>[2x]GMIKQDVICYEKEDVVKRNNINITGGGEKTVLLAHGFGCDQNMWRFMLPELEKQFTVIVFDYVGSGQSDLESFSTKRYSSLEGYAKDVEEILVALDLVNVSIIGHSVSSIIAGIASTHVGDRISDITMICPSPCFMNFPPDYVGGFERDDLEELINLMDKNYIGWANYLAPLVMGASHSSELIGELSGSFCTTDPIVAKTFAKATFFSDYRSLLEDISTP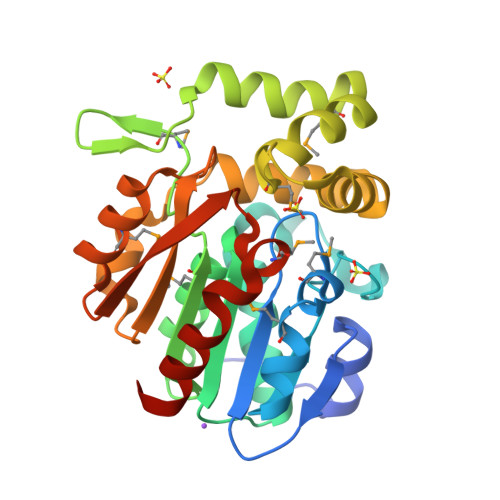ALIFQSAKDSLASPEVGQYMAENIPNSQLELIQAEGHCLHMTDAGLITPLLIHFIQNNQTRA>MSTVVQQVPAELQAALTLINNDPRMRTNNAWALSADKRWSLKFTAELSVPCSSFMPDNSVWHLVLWQEETLIRIEVYPDKSEGISATFQHQNYNFSDASTREWTSGNPALENTPTVFGRNLWGLEPEALLDRISWRLSRLLLWIDAAAQEKLATTGDAVELPAFPDQSPFTVIGFSEQIDDLPFWASKTGEWGFASSTGLPGAHGTLFLREFLDNKGKLIRTTKWSPFMRKGARTTNAVWSVLPTLPVLAPWQAPRTWQELSHCFAQCGLSLPDLFSDIGRSVRALRKQRAPGLLLLGFPLENKIGDEPARIHWLALRLAGLSNTMTKRPGFRPTERNRRTWDREQPLSQEPIRWVRTQNWAADQLRTRGEAANDIRSKKVLIIGAGSLGSMIAENLMRIGVVSQGILDADLLQTGNLSRHALTMTSVGHNKAAALVEHLNRILPDASARSFSCAFPPESEVAKNSLRQYDVIIDCTGDDGVLKSLAAFDWKSEKIFISLAMTWRAEGLFAFAASETSFPVTDASSRFNASASPEIDMDEARIEGIGAWHPVFPARADDVQLWAAVGTKFICRVVSAPGRIYEYFKQMPDGTVEKEPHEY[2x];> MKSSHHHHHHENLYFQSNAELQPQFNEFLAN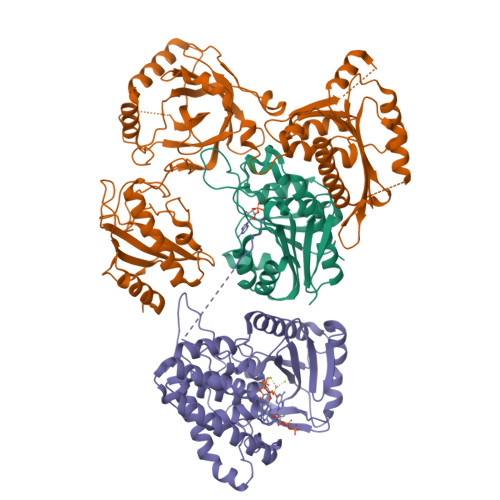IRPTDTQKEDWKSGARTLRERLKNFEPLKEIVVSTFLQGSIRRSTAIRPLGDKRPDVDIVVVTNLDHTRMSPTDAMDLFIPFLEKYYPGKWETQGRSFGITLSYVELDLVITAIPESGAEKSHLEQLYKSESVLTVNSLEEQTDWRLNKSWTPNTGWLSESNSAQVEDAPASEWKAHPLVLPDREKNEWGRTHPLAQIRWTAEKNRLCNGHYINLVRAVKWWRQQNSEDLPKYPKGYPLEHLIGNALDNGTTSMAQGLVQLMDTFLSRWAAIYNQKSKPWLSDHGVAEHDVMARLTAEDFCSFYEGIASAAEIARNALASEEPQESAQLWRQLFGSKFPLPGPQGGDRNGGFTTPSKPAEPQKTGRFA Fructosyl peptide oxidases (FPOX) are deglycating enzymes that find application as key enzymatic components in diabetes monitoring devices. The inability of wild type FPOXs to act on intact proteins is the most critical issue limiting both their diabetes detection efficiency and their protein deglycation potential. This is due to their buried active site and narrow access tunnel, as determined in multiple crystal structures. In that account, using a rational design approach involving a five-amino acid deletion at the entrance of the active site and a number of further mutations, we described a stable PnFPOX mutant (named L3-35A) that, relative to the wild type enzyme, features a significantly wider and shorter access tunnel.

In the present study, we set out to enhance the thermal stability of the L3-35A mutant by implementing a methodological approach whereby different thermal stabilization strategies are tested in parallel and their efficiency compared. These various strategies involved mutations to either improve the RMSF of the protein (generating mutants hereafter referred to as D-series mutants), increase the number of salt bridges (C-series mutants) or form disulfide bonds (X-series mutants). Our MD-based ranking led to the selection of six candidate mutants (C16, D02, X01, X02A, X04, and X07) for experimental production and characterization. On the other hand, the introduction of extensive surface charges and salt bridges (mutant C16) resulted in a further increase in Tm of ≈ 1.5 °C (Tm = 55.2 °C). Finally, the incorporation of a single disulfide bond in different positions on the L3-35A scaffold led to a significant improvement in thermal stability of all the tested mutants of this series: X01 (54.1 °C), X02 (60.0 °C), X04 (55.2 °C) and X07 (55.3 °C). In particular, we have shown that the introduction of a disulfide bond allowed us to produce a PnFPOX variant that shows remarkably higher thermal stability compared to the other mutants. We observed that the activity of the enzyme variants towards fK and fV remained similar to that of the parent enzyme, with a slight increase of activity in the case of D02 and a slight decrease in all the other cases. Overall, we observed that the activity of these mutant enzymes is several folds lower than that of PnFPOX, the naturally occurring enzyme. Also, similarly to the parent enzyme, none of these mutants shows any activity towards the dipeptide or the hexapeptide. In this process, while the amino acids that are directly involved in the catalytic function were not modified, some tunnel-lining residues were replaced.

> APSRANTKVIVVGGGGTIGSSTALHLVRSGYTPSNVTVLDAYPIPSSQSAGNDLNKIMDADADPAADAARQMWNEDELFKKFFHNTGRLDCCHGEKDIADCKKRYQNLVDWGLDATVEWLDSEDEILKRMPQLTRDQIKGWKAIFSKDGGWLAAAKAIKAIGEYLRDQGVRFGFYGAGSFKQPLLAEGVCIGVETVDGTRYYADKVVLAAGAWSPTLVELQEQCVSKAWVYGHIQLTPEEAARYKNSPVVYNGDVGFFFEPNEHGIIKVCDEFPGFTRFKMHQPFGAKAPKRISVPRSHAKHPTDTIPDASIVRIRRAIATFMPQFKNKPLFNQAMCWCTDTADGHLLICEHPEWKNFYLATGDSGDSFKLLPIIGKYVVELLEGTLADELAHKWRWRPGSGDALKSRREAPAKDLADMPGWNHDH> MSLGAKPFGEKKFIEIKGRRMAYIDEGTGDPILFQHGNPTSSYLWRNIMPHCAGLGRLIACDLIGMGDSDKLDPSGPERYTYAEHRDYLDALWEALDLGDRVVLVVHDWGSVLGFDWARRHRERVQGIAYMEAVTMPIEWADFPEQDRDLFQAFRSQAGEELVLQDNVFVEQVLPGLILRPLSEAEMAAYREPFLAAGEARRPTLSWPRQIPIAGTPADVVAIARDYAGWLSESPIPKLFINAEPGHLTTGRIRDFCRTWPNQTEITVAGAHFI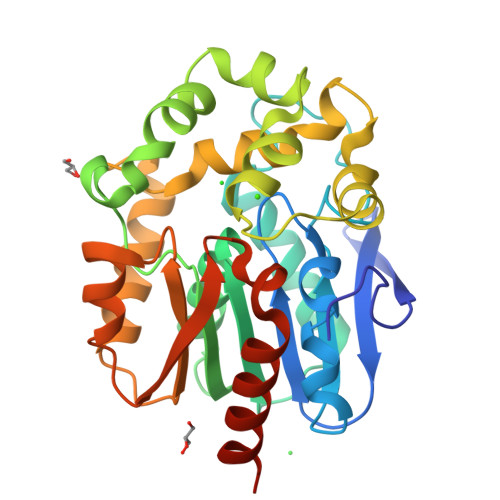QEDSPDEIGAAIAAFVRRLRPAHHHHHH As a proof of concept, we used this platform to identify both known and novel L- and D-amino acid peptide binders to the well-characterized model target, streptavidin. All peptides bind within or near the biotin binding pocket of streptavidin formed by two surface loops [1/2 (amino acids 22–28) and 3/4 (amino acids 42–52)], and by antiparallel β-sheets involved in an extensive polar interaction network, in which residues Ser88 and Thr90 of β-strand 6 play a major role. The surface loops of streptavidin are flexible: upon biotin binding they undergo a conformational change to form a closed conformation, but to accommodate the peptide ligands, loop 3/4 is dislocated by 13–16 Å from the biotin closed form to adopt a well-defined peptide-specific structure. All eight L- and D-peptides discovered in this work bind to the same pocket of streptavidin in distinctive binding modes suggesting (1) the rich malleability of L- and D-peptides and (2) the ability of streptavidin itself to adjust the flexible loop to accommodate multiple peptides with diverse sequences and conformations.

The same stepwise evolution approach was followed to identify hotspot D-amino acid sequences that bind to streptavidin. Two 5-mer hotspots, “wqeea” and “lanvd”, were selected for the extension step with all 160,000 possible combinations of D-amino acid dimers. All D-peptides fold into a left-handed α-helix with one turn for GyGlanvdessG and two turns each for the Gdlwqheatwkkq and GGwhdeatwkpG peptides.

>[4x]MRKIVVAAIAVSLTTVSITASASADPSKDSKAQVSAAEAGITGTWYNQLGSTFIVTAGADGALTGTYESAVGNAESRYVLTGRYDSAPATDGSGTALGWTVAWKNNYRNAHSATTWSGQYVGGAEARINTQWLLTSGTTEANAWKSTLVGHDTFTKVKPSAASIDAAKKAGVNNGNPLDAVQQ;>GYGLANVDESSG[3x]>GPETLCGAELVDALQFVCGDRGFYFNKPKAKGIVDECCFRSCDLRRLEM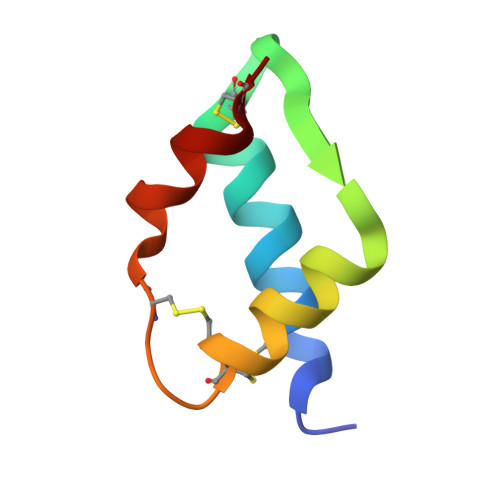YCA[2x]> KFSAKRLPSTRLGTFLENRVNDFLRRQNHPESGEVTVRVVHASDKTVEVKPGMKARFVDSGEMAESFPYRTKALFAFEEIDGVDLCFFGMHVQEYGSDCPPPNQRRVYISYLDSVHFFRPKCLRTAVYHEILIGYLEYVKKLGYTTGHIWACPPSEGDDYIFHCHPPDQKIPKPKRLQEWYKKMLDKAVSERIVHDYKDIFKQATEDRLTSAKELPYFEGDFWPNVLEESIKELEQEEEERKREENTSNESTDV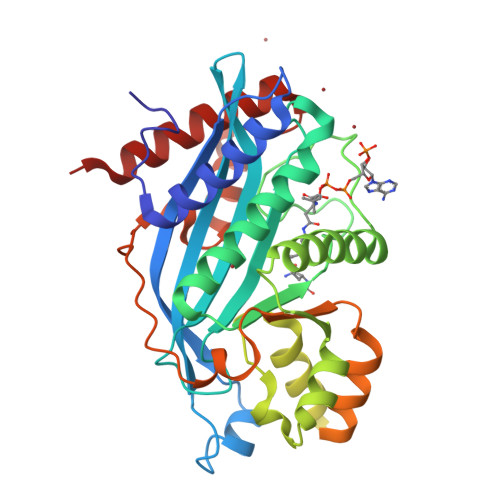TKGDSKNAKKKNNKKTSKNKSSLSRGNKKKPGMPNVSNDLSQKLYATMEKHKEVFFVIRLIAGPAANSLPPIVDPDPLIPCDLMDGRDAFLTLARDRHLEFSSLRRAQWSTGCMLVELHTQSQDRF ATAs transfer an amino group of a chiral amine compound to a ketone compound using the cofactor pyridoxal 5’-phosphate (PLP) with a high turnover rate, stable catalytic activity, broad substrate specificity and excellent stereoselectivity, which is achieved by a proposed large-binding pocket (L pocket) and small-binding pocket (S pocket) in the substrate-binding site8910111213141516. Each protomer (subunit) of the dimeric enzymes shows a structural architecture typical of the fold-type IV class of PLP-dependent enzymes, which are made up of two domains. The substrate-binding site is surrounded by the cavity among the two domains, the cofactor PLP, and the loop consisting of the residues 129–145 of the other protomer. The substrate-binding site can be divided into two parts as described initially, the L pocket and the S pocket, which is consistent with the previously proposed mechanism for the substrate specificity of ATAs in which the smaller and larger atomic groups of substrates are recognized by the S and L pockets, respectively.

The first R-ATA, which was identified from Arthrobacter sp. KNK168 (FERM-BP-5228) (Ab-R-ATA) by enrichment screening, showed activity on primary amine and methyl ketones or small cyclic ketones. In this study, we used Ab-R-ATA instead of ATA-117, the parental enzyme of ATA-117-Rd11, and could elucidate a reasonable molecular mechanism underlying the engineering of ATA-117-Rd11 because the difference between Ab-R-ATA and ATA-117 is only the amino acid residue at position 306 (Val and Ile in Ab-R-ATA and ATA-117, respectively) far from the active site, which is supposed to have negligibly small effect on the substrate recognition and activity and is not conserved in R-ATAs. The models complexed with a glycerol molecule at the active site of Ab-R-ATA suggested that Arg138 of the wild-type Ab-R-ATA is important for the recognition of probable native substrates, such as pyruvate. The kcat/Km values for pyruvate of the R138A and the R138Q mutants, using (R)-1-phenylethylamine as the amino donor, were about 350-fold and 500-fold lower than that of the wild-type Ab-R-ATA, respectively, indicating that the side chain of Arg138 is important for the recognition of pyruvate. The importance of Arg138 in the pyruvate recognition was also supported by molecular dynamics (MD) simulations of the wild-type Ab-R-ATA complexed with PMP-pyruvate quinonoid intermediate. During the simulation, the carboxyl group of the quinonoid intermediate formed a stable salt bridge with guanidinium group of Arg138. Although the corresponding arginine residue is not conserved in Ab-R-ATA, the guanidinium group of Arg138 of Ab-R-ATA was located near the position where the guanidinium groups of those arginine residues in the other R-ATAs.

> MAFSADTSEIVYTHDTGLDYITYSDYELDPANPLAGGAAWIEGAFVPPSEARISIFDQGYLHSDVTYTVFHVWNGNAFRLDDHIERLFSNAESMRIIPPLTQDEVKEIALELVAKTELREAFVSVSITRGYSSTPGERDITKHRPQVYMYAVPYQWIVPFDRIRDGVHAMVAQSVRRTPRSSIDPQVKNFQWGDLIRAVQETHDRGFEAPLLLDGDGLLAEGSGFNVVVIKDGVVRSPGRAALPGITRKTVLEIAESLGHEAILADITLAELLDADEVLGCTTAGGVWPFVSVDGNPISDGVPGPITQSIIRRYWELNVESSSLLTPVQY>[2x]MEMTEYRQCVAKPISSSNPVGERLVDHPLFDFIEDQMMKVGSLSHASVQWDEVEHSTLKLLGEQSKDIKLLVYLLQCLHNQVTPTRLITSFAVMSEFLNQYWNDSYPAPGARGNLPRRKFFSQMAQRFTTVIEKFDFHHLDEADRQALQAAVEEWQQAVEKQGLSSELVESVVVRITAEIKRAEQRQQVTAQSSAERETPSAATSSPAASMVVDHSSDKAAKQTLLKVADFLAEQEFGIALSIRLRRFAVWGSITSLPDHKPDGETLLRGMQADRVKDYQDQLRHPDLALWRKVEQSLTMAPYWFEGQWMSYTIAQQLGKSDWCQAIAEETQQFLRRLPSLLELKFKGGEPFVSDSVKEWLASVGQSQGAAGQSVGGDWQEKRKEAFQLAKEGGIAVALSMLNDGLVSAVEPRDKFYWRLLSADLLRANHLDAMAGEQYQTLLNQVTTLSVPEWEPSLVEQIQRYTTSE

The type VI secretion system (T6SS) is a membrane‐anchored contractile nanomachine used by many Gram‐negative bacteria to deliver proteins from the cytosol directly to an extracellular space or across a target cell membrane. All TssA‐like proteins harbor a conserved ImpA_N domain (PF06812) located at the N‐terminal end, while the C‐terminal part differs in its composition. The Vibrio cholerae and P. aeruginosa TssA proteins TssAVC and TssA2PA with C‐terminal VasJ domain (Class A) facilitate sheath assembly initiation and polymerization by forming a stable dodecamer at the end of the sheath that is distal from the membrane anchor. Therefore, while potentially not being strictly essential, Class A TssAs act as chaperones assisting sheath‐tube copolymerization, which likely requires assistance in proper formation of the sheath hand‐shake domain (Ge et al, 2015; Kudryashev et al, 2015; Wang et al, 2017).

To further analyze the TssA of V. cholerae, we purified the protein and used cryo‐electron microscopy (cryo‐EM) to solve its structure. To test the symmetry, an initial 3D reference was built and refined without imposing any symmetry (C1), which resulted in clear six‐pointed star reconstruction. Further refinements have been done utilizing C6 symmetry. The outer and lumenal diameters are 132 and 53 Å, and the height of the assembly is 38 Å. Molecular weight estimation from the size‐exclusion chromatography (SEC) profile is ~600 kDa, which corresponds to twelve copies of TssAVC in one oligomer (634 kDa from sequence). The model built in cryo‐EM density of TssAVC is composed of twelve C‐terminal subunits (G376‐T466, helices α8–α12) tightly packed as two interpenetrating rings, similar to A. hydrophila TssA (TssAAH), but different from head‐to‐head stacked hexameric rings of the TssAEC assembly (Zoued et al, 2016; Dix et al, 2018). Each of the C‐terminal subunits forms two interfaces with its neighbors. The first 688 Å2 PISA‐predicted interface is based on three conserved residues (W454, E455, and P456) from α11–α12 linker of one subunit and helix α10 from the neighboring subunit. Second 672 Å2 interface forms a sixfold axis between helices α9–α11 of two neighboring subunits. Our reconstruction of TssAVC CTD fits as a rigid body with CC = 0.87 into the distal end of VipA‐N3 sheath mutant reconstruction.> MSFTNATFSQVLDDLSARFILNLPAEEQSSVERLCFQIEQAHWFYEDFIRAQNDQLPSLGLRVFSAKLFAHCPLLWKWSKVHEEAFDDFLR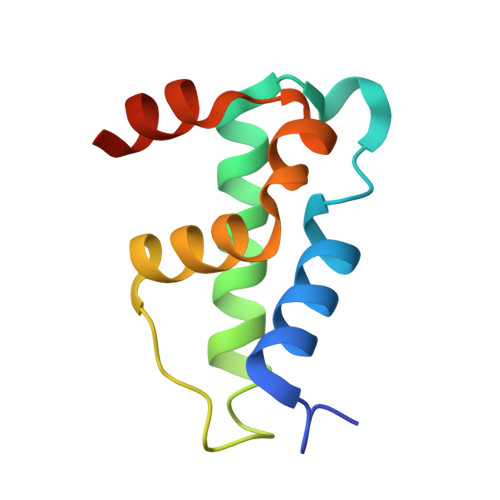YKTR> MDPIALQAGFDLLNDGRPETLWLGIGTLLMLIGTFYFIARGWGVTDKEAREYYAITILVPGIASAAYLAMFFGIGVTEVELASGTVLDIYY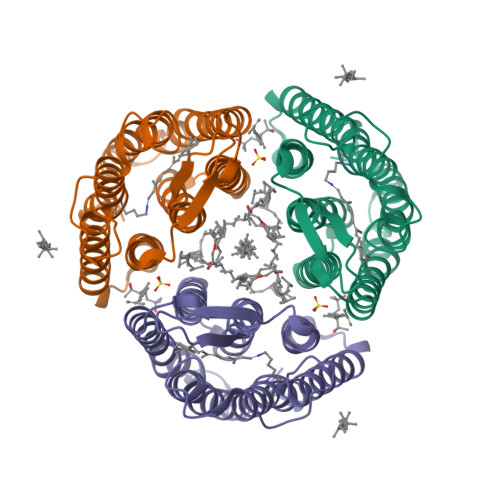ARYADWLFTTPLLLLDLALLAKVDRVTIGTLIGVDALMIVTGLIGALSKTPLARYTWWLFSTIAFLFVLYYLLTSLRSAAAKRSEEVRSTFNTLTALVAVLWTAYPILWIVGTEGAGVVGLGIETLAFMVLDVTAKVGFGFVLLRSRAILGETEAPEPSAGADASAAD>[9x]GPHMSVSFRDRVLKLYLLGFDPSEIAQTLSLDAKRKVTEEEVLHVLAEARELLSALPSLEDIRAEVGQALERARIFQKDLLAIYQNMLRNYNAMME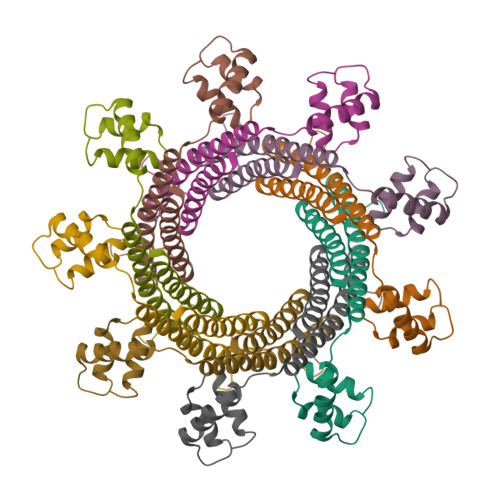GLTEHPDGTPVIGVRPADIAAMADRIMKIDQERITALLNSLKVLGHVGSTTAGALPSATELVSVEELVAEVADETPKT>ASLTEIEHLVQSVCKSYRETCQLRLEDLLRQRSNIFSREEVTGYQRKSMWEMWERCAHHLTEAIQYVVEFAKRLSGFMELCQNDQIVLLKAGAMEVVLVRMCRAYNADNRTVFFEGKYGGMELFRALGCSELISSIFDFSHSLSALHFSEDEIALY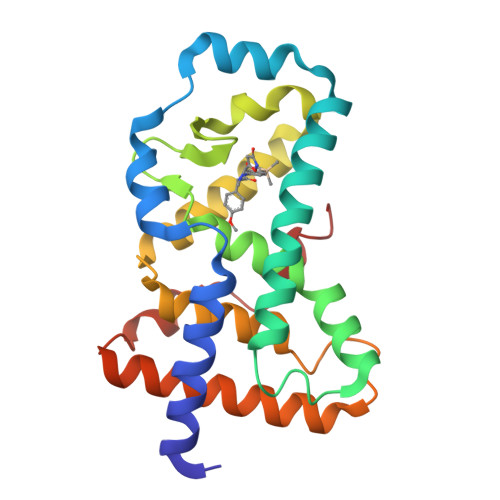TALVLINAHRPGLQEKRKVEQLQYNLELAFHHHLCKTHRQSILAKLPPKGKLRSLCSQH[2x]> MQLGQLRQPLRACQDQRLTRGVPLARRQLVVVSNWNPLGGKGGGNAEQPGGEEPIQDELLKLLRGGWVLLSNLALFLVFSSFLHRSLNWFVQTELLVAVGAPQQAGERVVGKFFEAIEWVERNILGWKLPGDEEAEDATSKVYEVLQNYTPAEAAYSFAQLKYKDLTHKERELFHKAYALRHFERRDGRPGDVDAAELQAVKDRLD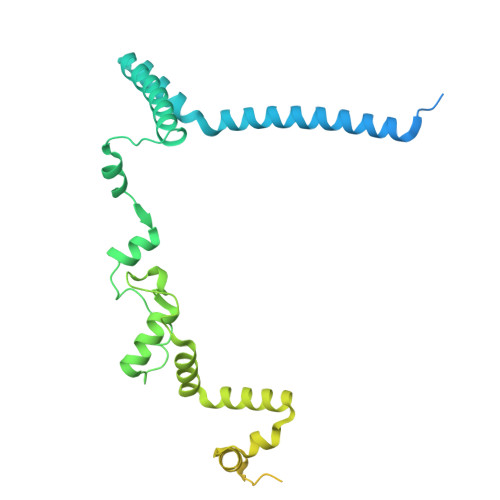PLEADRRAYAAAKAAGRLDEYWAAPGREATYQRIVGAPRIAARQCEMASMLKGLQAVLPAMELLAQLQVAQFVYAASKASKSRQQDDFKLQLQTFYGNVLDEQCQLRCMLLNVQLPMALVTVFVPQYCFCLLDRVVLPRRECGSASTLGSLLRACGRPGSACHAGGCSAQRRDPLTI> GFSSEDKGEWKLKLDNAGNGQAVIRFLPSKNDEQAPFAILVNHGFKKNGKWYIETCSSTHGDYDSCPVCQYISKNDLYNTDNKEYSLVKRKTSYWANILVVKDPAAPENEGKVFKYRFGKKIWDKINAMIAVDVEMGETPVDVTCPWEGANFVLKVKQVSGFSNYDESKFLNQSAIPNIDD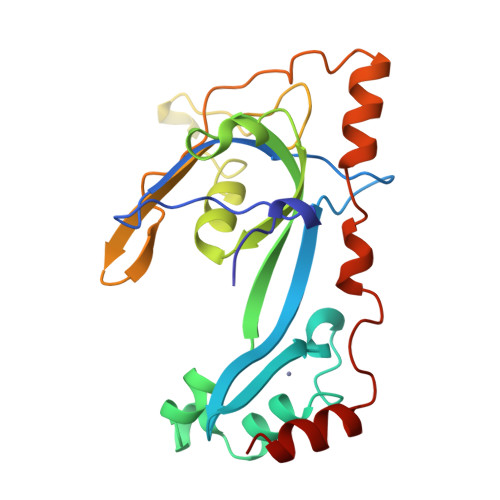ESFQKELFEQMVDLSEMTSKDKFKSFEELNTKFGQVM> PPFRFKAPQEVRIKVPIGRIPPAVGPEIRLGKSIVAVAPHRVTAEQLEDARRVLRRVLGRSKEVHQNVHATYAVTRKPEGTKMGQGKG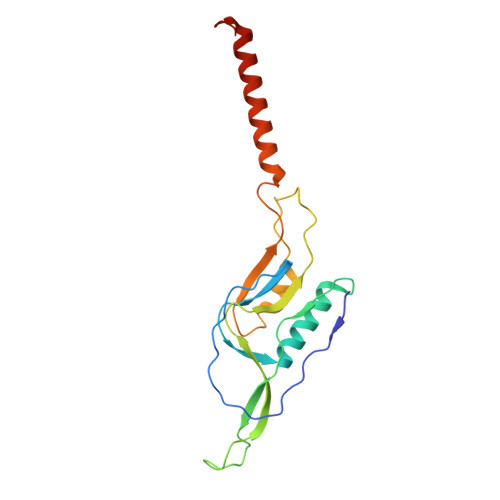SIDRFVARVPAGRILFHIPQINPFHPFPEVEPNFAAFKAIAPRLPVPVVFREQNNFFQMHSVKDLIRKRQAEERENREKTARDKLGGFHTD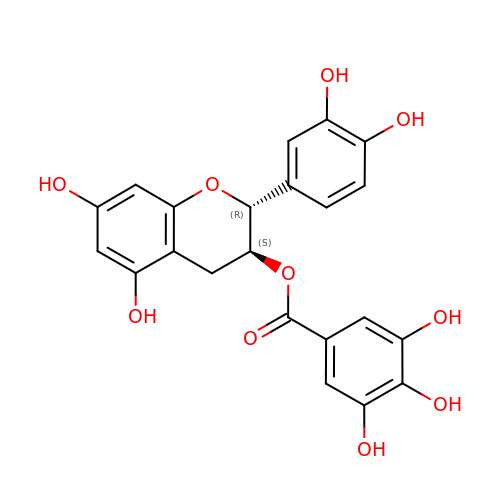(2R,3S)-2-(3,4-dihydroxyphenyl)-5,7-dihydroxy-3,4-dihydro-2H-chromen-3-yl 3,4,5-trihydroxybenzoate | C22 H18 O10 | LSHVYAFMTMFKBA-PZJWPPBQSA-N>X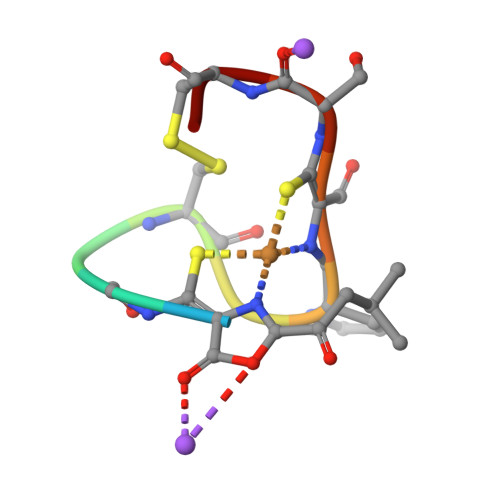CGSCYPCSCM[2x]> MPPQLHNGLDFSAKVIQGSLDSLPQEVRKFVEGNAQLCQPEYIHICDGSEEEYGRLLAHMQEEGVIRKLKKYDNCWLALTDPRDVARIESKTVIITQEQRDTVPIPKSGQSQLGRWMSEEDFEKAFNARFPGCMKGRTMYVIPFSMGPLGSPLAKIGIELTDSPYVVASMRIMTRMGTSVLEALGDGEFIKCLHSVGCPLPLKKPLVNNWACNPELTLIAHLPDRREIISFGSGYGGNSLLGKKCFALRIASRLAKEEGWLAEHMLILGITNPEGKKKYLAAAFPSACGKTNLAMMNPTLPGWKVECVGDDIAWMKFDAQGNLRAINPENGFFGVAPGTSVKTNPNAIKTIQKNTIFTNVAETSDGGVYWEGIDEPLAPGVTITSWKNKEWRPQDEEPCAHPNSRF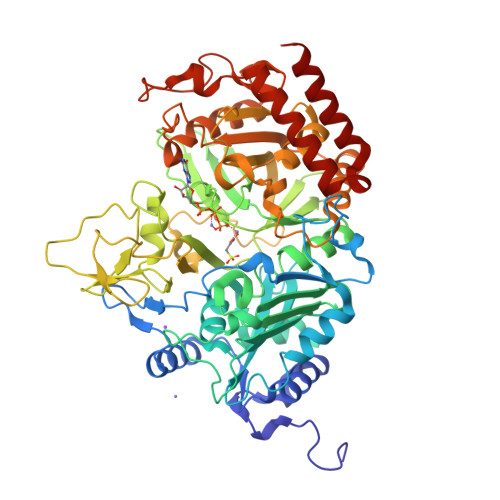CTPASQCPIIDPAWESPEGVPIEGIIFGGRRPAGVPLVYEALSWQHGVFVGAAMRSEGGIMHDPFAMRPFFGYNFGKYLAHWLSMAHRPAAKLPKIFHVNWFRKDKNGKFLWPGFGENSRVLEWMFGRIEGEDSAKLTPIGYVPKEDALNLKGLGDVNVEELFGISKEFWEKEVEEIDKYLEDQVNADLPYEIERELRALKQRISQM>MDSTEAEQMDTEQATNQTAEAGGGGGGGGGGGGGGGGVGNSTGGFNNTTEFKVINNEVYITCHATRMVHINQADTDEYLIFNAGRTTDTKTHQQKLNLEFFVYDDFHQQVMTPWYIVDSNAWGVWMSPKDFQQMKTLCSEISLVTLEQEIDNVTIKTVTETNQGNASTKQFNNDLTASLQVALDTNNILPYTPAAPLGETLGFVPWRATKPTQYRYYHPCYIYNRYPNIQKVATETLTWDAVQDDYLSVDEQYFNFITIENNIPINILRTGDNFHTGLYEFNSKPCKLTLSYQSTRCLGLPPLCKPKTDTTHKVTSKENGADLIYIQGQDNTRLGHFWGEERGKKNAEMNRIRPYNIGYQYPEWIIPAGLQGSYFAGGPRQWSDTTKGAGTHSQHLQQNFSTRYIYDRNHGGDNEVDLLDGIPIHERSNYYSDNEIEQHTAKQPKLRTPPIHHSKIDSWEEEGWPAASGTHFEDEVIYLDYFNFSGEQELNFPHEVLDDAAQMKKLLNSYQPTVAQDNVGPVYPWGQIWDKKPHMDHKPSMNNNAPFVCKNNPPGQLFVKLTENLTDTFNYDENPDRIKTYGYFTWRGKLVLKGKLSQVTCWNPVKRELIGEPGVFTKDKYHKQIPNNKGNFEIGLQYGRSTIKYIY[60x]

Aleutian mink disease virus (AMDV), a pathogen in minks, and human parvovirus 4 (PARV4), infecting humans, are parvoviruses belonging to the genera Amdoparvovirus and Tetraparvovirus, respectively. Despite low amino acid sequence identities (10–30%) both viruses share the icosahedral nature of parvovirus capsids, with 60 viral proteins (VPs) assembling the capsid via two-, three-, and five-fold symmetry VP-related interactions, but display major structural variabilities in the surface loops when the capsid structures are superposed onto other parvoviruses. The viral capsids are critical components of the viral infectious life cycle: they protect the viral genome, are the determinants of the tissue type and host that is targeted (tropism), and remain intact while the virus escapes the endo-/lysosomal pathway and trafficks to the nucleus where the genome is released, leading to viral genome replication. The VP monomers of PARV4 and AMDV conserve the β-barrel core motif (βB–βI) with the additional βA strand and the α-helix A (αA) observed in other parvoviruses.

Three-dimensional-image reconstruction of a total of 93,393 individual AMDV capsids resulted in a resolution of 2.37 Å, based on an FSC threshold of 0.143. The reconstructed capsid of AMDV, the first determined structure of the genus Amdoparvovirus, also displayed familiar surface features with channels at the icosahedral five-fold axes, protrusions near the three-fold axes, and depressions at the two-fold axes and surrounding the five-fold axes. Unlike PARV4, the three-fold protrusions were separated and radiated further outwards (the maximum capsid diameter of AMDV being ~300 Å compared to ~270 Å for PARV4). The amino acids, including their side chains in the VP monomers, were generally very well-ordered to the C-terminal tyrosine 647, with the exception of the apexes of the loops at the three-fold protrusion, involving aa 93–94 and 238–239, which showed only weak density at a sigma (σ) threshold of ~1, preventing reliable placement of the amino acid side chains. However, due to the cleavage of the AMDV VPs at D420, no density was observed for aa 420 to 449, but both ends of VR-VII, leucine 419 and proline 450, were visible at the capsid surface. However, in contrast to PARV4, the elongated VR-I and VR-III (15 and 18 aa longer, respectively) are responsible for the three-fold protrusions in AMDV. The region at the three-fold symmetry axis between the protrusions is primarily formed by VR-VIII, while VR-V is not surface-exposed. The VR-VIII loop possesses an additional α-helix B. In fact, three helices from three symmetry-related VPs are positioned around the three-fold symmetry axis, creating a small pore with a diameter of ~3.5 Å. In fact, AMDV has the longest loop for VR-I, VR-III, VR-IV, and VR-VII among natural Parvovirinae isolates for which structures have been determined.>MPKYAPHVYTEQAQIATLEHWVKLLDGQERVRIELDDGSMIAGTVAVRPTIQTYRDEQEREGSNGQLRIDHLDASQ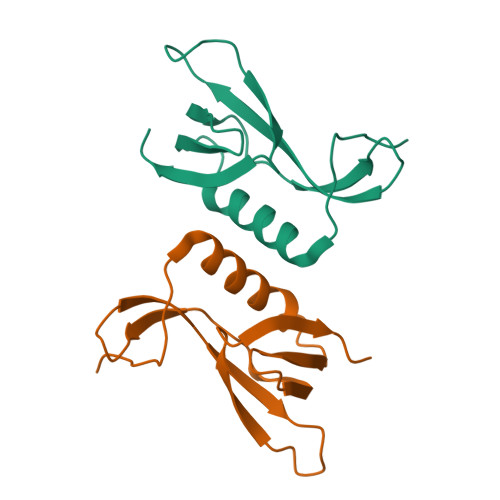EPQWIWMDRIVAVHPMPLGAPQVMP[2x]>[2x]MSEEQSHADQDAYVADVDGILDVLRAQVLERKPDDIFQFISKSALSLQKDRGAESCDRINCKVKDEQKSRALTIIVFGASGDLAKKKTFPALFDLYCGGLLPPEVNIIGYARTKVDDVEKWKHETLMKYFSNLSERGCHAEDFLKHISYFCGAYDSVDDFKRLDAVIREKENAFKGPEKGGNRLFYLALPPSVFASVCESIHKGAMPQEVGGWVRVIIEKPFGRDTKSSAELSQALEPFFDESQLYRIDHYLGKEMVQNIITTRFANRIFSAVWNASNIACVQITFKETIGTEGRGGYFDNIGIIRDVMQNHLTQILALLAMEKPRSLDAECIRDEKVSVLKCIEPITKENCVLGQYTASADGSIPGYLEDVTVPEGSTCPTFAVMRLNINNDRWAGVPFILKAGKAVEQKYVAIRIQFRDEVHPYGEATQRNELVIRAQPSEAMYVKITTKVPGLSGDLRQTHQTELDLTYHTRYDVRLPDAYESLINDALLGNSTNFVRKDELDVAWRIFTPLLHQIDSGEIKPIPYQAGTRGPKEADEFIANNGFKHQKGYHWLPSNKL

The housekeeping enzyme glucose 6-phosphate dehydrogenase (G6PD) (EC 1.1.1.49) is the first and rate-limiting enzyme of the PPP. It catalyzes the oxidation of glucose 6-phosphate (G6P) originating from glycolysis to 6-phospho-D-glucono-1,5-lactone (6PL), whereby the cofactor NADP+ is reduced to NADPH. In the present study, we describe the crystal structures of Leishmania donovani G6PD (LdG6PD), both native and complexed with one or both substrates. The LdG6PD monomer contains three domains: an N-domain (Q5-K49), the NADP+ binding “Rossmann-like” domain (residues D50-I248), and a β + α domain (residues D249-K552).

In contrast, the LdG6PD wt and the LdG6PDC138S mutant, complexed with NADP(H), G6P, or both substrates, adopt C121 space group symmetry with one dimer in the AU (AB). Crystals containing only NADP(H) diffracted to a resolution up to 1.7 Å, and crystals containing G6P or G6P and NADP(H) to 3.3 Å and 2.5 Å, respectively. Comparing the apo structure with the structures complexed with G6P, NADP(H) or both substrates reveals a rotation of the N-domain by about 45° upon ligand binding. However, the described conformational changes upon NADP(H) binding did not extend to the NADP+ binding pocket. Moreover, the LdG6PD wt structure, complexed with NADP(H), revealed a disulfide bond between C138 and C56; however, with minor conformational changes, an alternative disulfide bond between C138 and C61 or C56 and C97 is also possible. Without bound G6P, the H250 and K254 side chains face away from the binding pocket, making the usual interaction with G6P impossible. Moreover, Y251 points into the G6P binding pocket, which would lead to clashes with the phosphate moiety of G6P in LdG6PD and homologous structures. Interestingly, NADP(H) is always visible in both monomers of the dimer, while G6P is visible in monomer B only. Therefore, structures complexed only with NADP+, were always crystallized under catalysis. Accordingly, the bound NADP+ could also be the product NADPH.Intracellular nucleotide binding, leucine-rich repeat (NLR) receptors are key components of plant innate immunity pathways. The integrated HMA domain in the sensor NLR Pik-1 directly binds the effector AVR-Pik. The Pikp NLR allele only responds to the effector variant AVR-PikD, but the Pikm allele responds to AVR-PikD, AVR-PikE, and AVR-PikA. Here, we graft an interface from Pikm onto Pikp by mutating two residues in Pikp (Asn261Lys, Lys262Glu), forming PikpNK-KE.

To this end, we determined the crystal structures of Pikp-HMANK-KE bound to AVR-PikD, and to AVR-PikE. Each complex was crystallized and X-ray diffraction data were collected at the Diamond Light Source (Oxford, UK) to 1.6 Å and 1.85 Å resolution, respectively. The overall architecture of these complexes is the same as that observed for all Pik-HMA/AVR-Pik effector structures. A key interaction at interface 3, one of the previously defined Pik-HMA–AVR-Pik interfaces, involves a lysine residue (Lys262 in Pikp and Pikm) that forms intimate contacts within a pocket on the effector surface. In order to position this lysine in the effector pocket, Pikp has to loop-out regions adjacent to this residue, compromising the packing at the interface (De la Concepcion et al., 2018, Figure 3A, B, C and D). In the PikpNK-KE mutant, the position of this key lysine is shifted one residue to the N-terminus compared to that in the wild-type, so that it occupies the same position in the PikpNK-KE sequence as in the Pikm sequence. In the crystal structures of Pikp-HMANK-KE in complex with either AVR-PikD or AVR-PikE, we see that this region of the HMA adopts a Pikm-like conformation (Figure 3A, B, C and D), with no looping-out of the preceding structure. The cell-death response to AVR-PikD mediated by PikpNK-KE is similar but elevated when compared to that mediated by Pikp.

> GPGLKQKIVIKVAMEGNNCRSKAMALVASTGGVDSVALVGDLRDKIEVVGYGIDPIKLISALRKKVGDAELLQVSQAKED;> METGNKYIEKRAIDLSRERDPNFFDHPGIPVPECFWFMFKNNVRQDAGTCYSSWKMDMKVGPNWVHIKSDDNCNLSGDFPPGWIVLGKKRPGF>SAMLLRFTKMHGLGNDFMVLDLVSQHAHVQPKHVKLWGDRNTGVGFDQLLIVEAPSSPDVDFRYRIFNADGSEVEQCGNGARCFARFVQDKRLTVKKSIRVETKGGIIELNIRPDGQVTVDMGPPRLAPAEIPFQAEREALSYEIEVNGQRVELAAVSMGNPHGVLRVENVD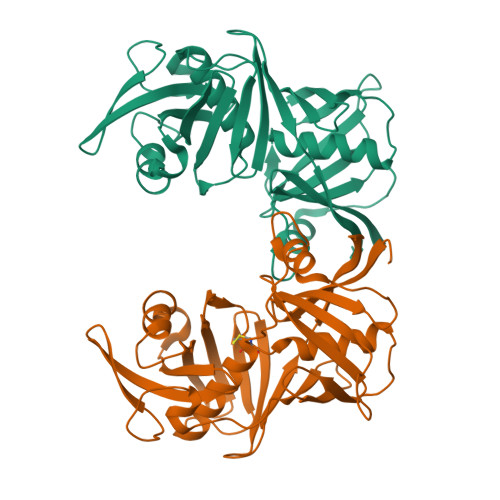SAPVHSLGPQLEVHPRFPKKANIGFLQVLDPHHARLRVWERGVGETQACGTGACAAAVAGIRQGWLQSPVQIDLPGGRLHIEWAGPGQPVMMTGPAVRVYEGQVRL[2x]> AHPLENAWTFWFDNPQGKSRQVAWGSTIHPIHTFSTVEDFWGLYNNIHNPSKLNVGADFHCFKNKIEPKWEDPISANGGKWTISCGRGKSDTFWLHTLLAMIGEQFDFGDEICGAVVSVRQKQERVAIWTKNAANEAAQISIGKQWKEFLDYKDSIGFI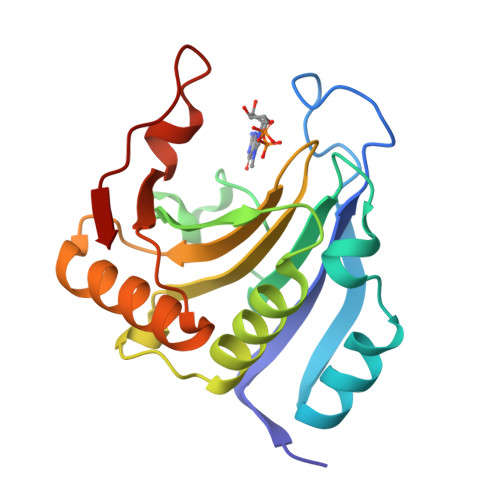VHEDAKRSDKGPKNRYTV>[2x]QTEQGANISDQWTGSELPLAFASDSNPSDPVSNVNDKLISYNNQPANRWTNWNRSNPEASVGVLFGDSGILSKRSVDNLSVGFHEDHGVGAPKSYVIEYYVGKTVPTAPKNPSFVGNEDHVFNDSANWKPVTNLKAPAQLKAGEMNHFSFDKVETYAIRIRMVKADNKRGTSITEVQIFAKQV

BgaA is specific for galactose β-1,4-linked to glucose or GlcNAc [lactose or N-acetyllactosamine (LacNAc) motifs, respectively] found in glycoconjugates. The N-terminal region of BgaA comprising amino acid residues 138–993 has amino acid sequence identity with GH family 2 enzymes. Through detailed structural and functional analyses the molecular basis for the catalytic specificity of BgaA is defined and this activity is demonstrated as critical for the ability of pneumococci to utilize complex N-linked glycans as a carbon source and protect the bacterium from opsonophagocytic killing. Further analyses also revealed the presence of non-catalytic CBMs within the C-terminal region of BgaA that mediate adherence to host cell surface LacNAc and/or lactose.

However, fold prediction using the Phyre2 server, which does not rely on amino acid sequence similarity, distinguished two regions (XII and XV) with a high probability of adopting the β-sandwich fold common to many CBMs found in CAZymes. The two predicted CBMs were recombinantly produced and the polypeptides screened for binding to all commonly occurring monosaccharides by UV difference spectroscopy; only D-galactose gave a signature UV difference spectrum consistent with sugar binding. Subsequently, this approach was expanded to the relevant galactose-containing sugars LacNAc, lactose, galactopyranosyl-β-1,3-N-acetyl-D-glucosamine (lacto-N-biose), and galactopyranosyl-β-1,3-N-acetyl-D-galactosamine [Thomsen-Freidenreich (TF) epitope] and binding was only observed to LacNAc and lactose. Significantly, the CBMs only bound with significant affinity to sugars that are substrates for the catalytic domain. A single bound metal ion was modeled as Ca2+ on the basis of coordination geometry and B-factor analysis. The shallow LacNAc binding site sits at the apex of the β-fold opposite the N- and C-termini. Tryptophan 1514 lies directly beneath the glycoside bond and coplanar with the disaccharide thus providing CH-π interactions with both pyranose rings and a higher affinity for β-linked disaccharides than for galactose alone. This binding site architecture accommodates lactose and LacNAc, but would limit the recognition of other sugars terminating in β-linked galactose.> MAYEKELDAAKKAASLAARLCQKVQKALLQSDVQSKSDKSPVTVADYGSQAVVSLVLEKELSSEPFSLVAEEDSGDLRKDGSQDTLERITKLVNDTLATEESFNGSTLSTDDLLRAIDCGTS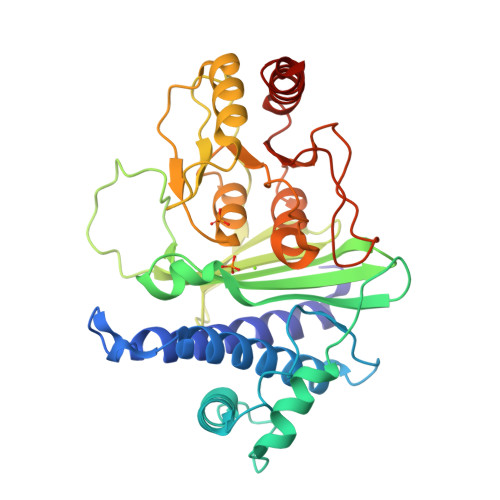EGGPNGRHWVLDPIDGTKGFLRGDQYAVALGLLEEGKVVLGVLACPNLPLASIAGNNKNKSSSDEIGCLFFATIGSGTYMQLLDSKSSPVKVQVSSVENPEEASFFESFEGAHSLHDLSSSIANKLGVKAPPVRIDSQAKYGALSRGDGAIYLRFPHKGYREKIWDHVAGAIVVTEAGGIVTDAAGKPLDFSKGKYLDLDTGIIVANEKLMPLLLKAVRDSIAEQEKASA>[2x]MQKPVCLVVAMTPKRGIGINNGLPWPHLTTDFKHFSRVTKTTPEEASRFNAVVMGRKTWESMPRKFRPLVDRLNIVVSSSLKEEDIAAEKPQAEGQQRVRVCASLPAALSLLEEEYKDSVDQIFVVGGAGLYEAALSLGVASHLYITRVAREFPCDVFFPAFPGDDILSNKSTAAEKDNEATYRPIFISKTFSDNGVPYDFVVLEKRRKTDDAATAEPSNAMSSLTSTRETTPVHGLQAPSSAAAIAPVLAWMDEE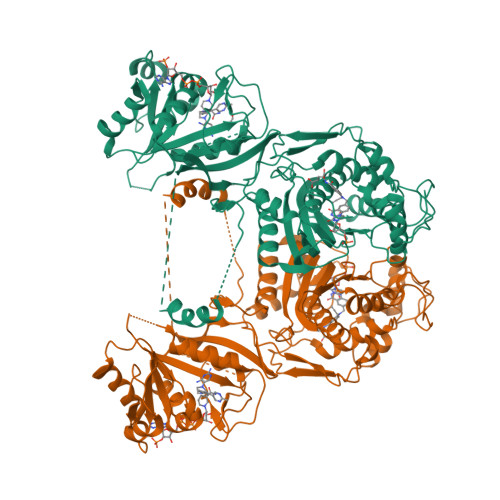DRKKREQKELIRAVPHVHFRGHEEFQYLDLIADIINNGRTMDDRTGVGVISKFGCTMRYSLDQAFPLLTTKRVFWKGVLEELLWFIRGDTNANHLSEKGVKIWDKNVTREFLDSRNLPHREVGDIGPGYGFQWRHFGAAYKDMHTDYTGQGVDQLKNVIQMLRTNPTDRRMLMTAWNPAALDEMALPPCHLLCQFYVNDQKELSCIMYQRSCDVGLGVPFNIASYSLLTLMVAHVCNLKPKEFIHFMGNTHVYTNHVEALKEQLRREPRPFPIVNILNKERIKEIDDFTAEDFEVVGYVPHGRIQMEMAV> MMKQALRVAFGFLILWASVLHAEVRIVIDSGVDSGRPIGVVPFQWAGPGAAPEDIGGIVAADLRNSGKFNPLDRARLPQQPGSAQEVQPAAWSALGIDAVVVGQVTPNPDGSYNVAYQLVDTGGAPGTVL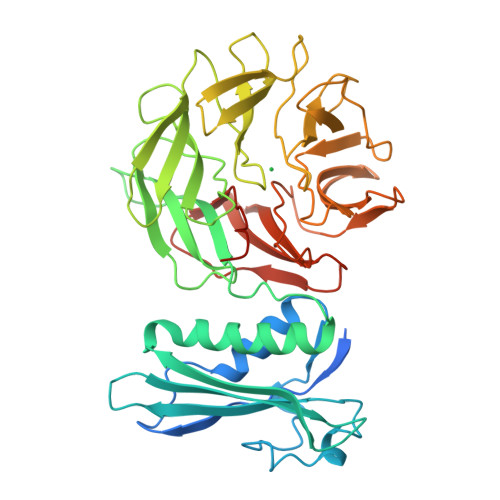AQNSYKVNKQWLRYAGHTASDEVFEKLTGIKGAFRTRIAYVVQTNGGQFPYELRVSDYDGYNQFVVHRSPQPLMSPAWSPDGSKLAYVTFESGRSALVIQTLANGAVRQVASFPRHNGAPAFSPDGSKLAFALSKTGSLNLYVMDLASGQIRQVTDGRSNNTEPTWFPDSQNLAFTSDQAGRPQVYKVNINGGAPQRITWEGSQNQDADVSSDGKFMVMVSSNGGQQHIAKQDLATGGVQVLSSTFLDETPSLAPNGTMVIYSSSQGMGSVLNLVSTDGRFKARLPATDGQVKFPAWSPYLLEHHHHHH> MARSMEQQEDSLEKVIKDT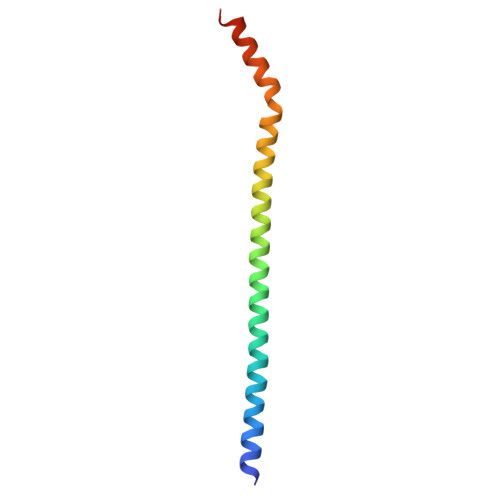ESLFKTREKEYQETIDQIELELATAKNDMNRHLHEYMEMCSMKRGLDVQMETCRRLITQSGDR> MASGGSGGVSVPALWSEVNRYGQNGDFTRALKTVNKILQINKDDVTALHCKVVCLIQNGSFKEALNVINTHTKVLANNSLSFEKAYCEYRLNRIENALKTIESANQQTDKLKELYGQVLYRLERYDECLAVYRDLVRNSQDDYDEERKTNLSAVVAAQSNWEKVVPENLGLQEGTHELCYNAACALIGQGQLSQAMKILQKAEDLCRRSLSEDSDGTEEDPQAELAIIHGQMAYILQLQGRTEEALQLYNQIIKLKPTDVGLLAVIANNIITINKDQNVFDSKKKVKLTNAEGVEFKLSKKQLQAIEFNKALLAMYTNQAEQCRKISASLQSQSPEHLLPVLIQAAQLCREKQHTKAIELLQEFSDQHPENAAEIKLTMAQLKISQGNISKACLILRSIEELKHKPGMVSALVTMYSHEEDIDSAIEVFTQAIQWYQNHQPKSSAHLSLIREAANFKLKYGRKKEAISDLEQLWKQNPKDIHTLAQLISAY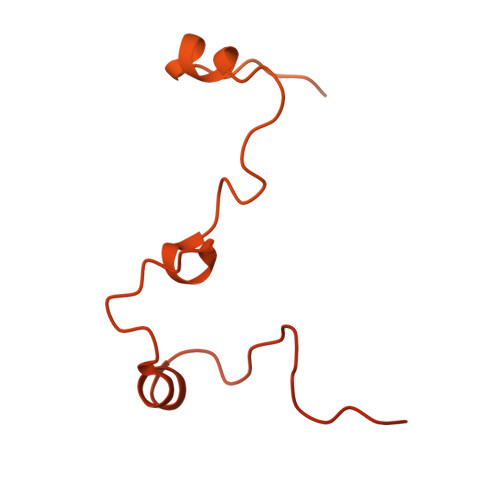SLVDPEKAKALSKHLPSSDSMSLKVDVEALENSPGATYIRKKGGKVAGDSQPKEQGQGDLKKKKKKKKGKLPKNYDPKVTPDPERWLPMRERSYYRGRKKGKKKDQIGKGTQGATAGASSELDASKTVSSPPTSPRPGSAATASASTSNIIPPRHQKPAGAPATKKKQQQKKKKGGKGGW>MPEIVDTCSLASPASVCRTKHLHLRCSVDFTRRTLTGTAALTVQSQEDNLRSLVLDTKDLTIEKVVINGQEVKYALGERQSYKGSPMEISLPIALSKNQEIVIEISFETSPKSSALQWLTPEQTSGKEHPYLFSQCQAIHCRAILPCQDTPSVKLTYTAEVSVPKELVALMSAIRDGETPDPEDPSRKIYKFIQKVPIPCYLIALVVGALESRQIGPRTLVWSEKEQVEKSAYEFSETESMLKIAEDLGGPYVWGQYDLLVLPPSFPYGGMENPCLTFVTPTLLAGDKSLSNVIAHEISHSWTGNLVTNKTWDHFWLNEGHTVYLERHICGRLFGEKFRHFNA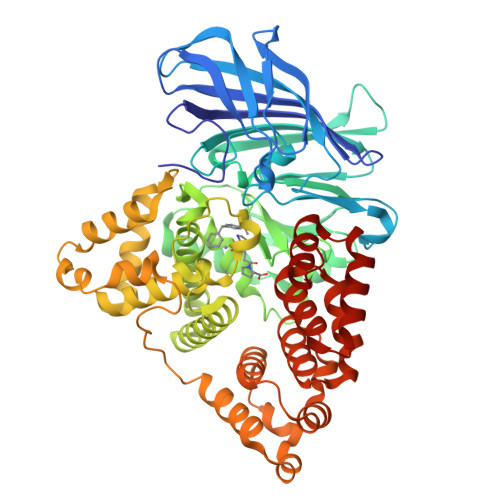LGGWGELQNSVKTFGETHPFTKLVVDLTDIDPDVAYSSVPYEKGFALLFYLEQLLGGPEIFLGFLKAYVEKFSYKSITTDDWKDFLYSYFKDKVDVLNQVDWNAWLYSPGLPPIKPNYDMTLTNACIALSQRWITAKEDDLNSFNATDLKDLSSHQLNEFLAQTLQRAPLPLGHIKRMQEVYNFNAINNSEIRFRWLRLCIQSKWEDAIPLALKMATEQGRMKFTRPLFKDLAAFDKSHDQAVRTYQEHKASMHPVTAMLVGKDLKVD[3x]>[2x]MAHHHHHHTMNIAKMIDHTLLKPEATEQQIVQLCTEAKQYGFAAVCVNPTWVKTAARELSGTDVRVCTVIGF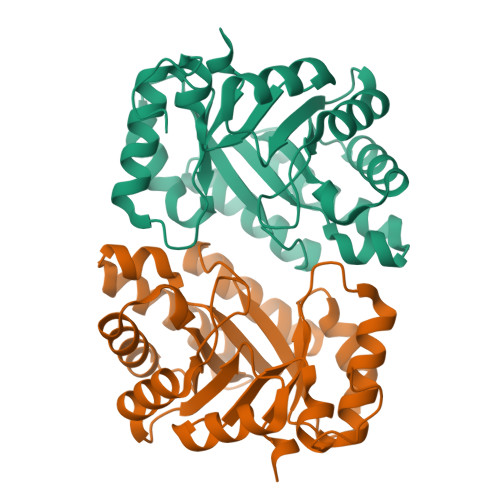PLGATTPETKAFETTNAIENGAREVDMVINIGALKSGQDELVERDIRAVVEAAAGRALVKVIVETALLTDEEKVRACQLAVKAGADYVKTSTGFSGGGATVEDVALMRKTVGDRAGVKASGGVRDWKTAEAMINAGATRIGTSSGVAIVTGGTGRADY Pralsetinib | C27 H32 F N9 O2 | 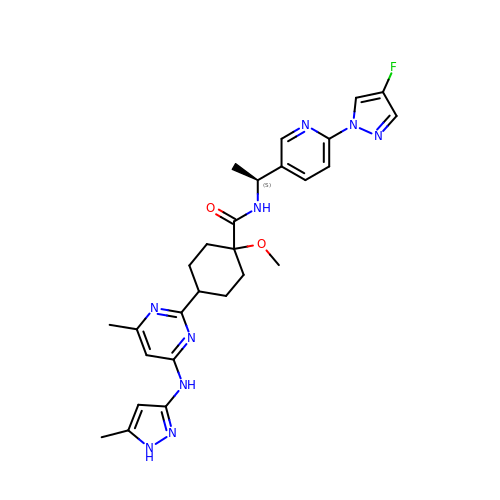GBLBJPZSROAGMF-BATDWUPUSA-N>MSDTSPGPEHAPAIDRLLQIATGFMASKVLLVAASLGLFTELAAGPLRGEELRARLRLHPRSARDFFDTLVALGVLERTNGAYANTPATAQYLVRGKSAYLGGLLEMSDARMYELWGRLDEGLRTGNPQNEIRTGEEGIYATLYDDPDRLDAFQQAMTGLSMRSAHALAEAIDWSAYRTVADIGCAEGTVLIHLLERHPHLRGTGFDLAAVRPSFQRRHEESGLGDRLAFRAGDFFAEPLPQADALVFGHILSNWALPKAKTLLRKAHEALPEGGIVVIYETLIDDERRENVPGLLMSLTMLLETPGGFEYTGADCREWLADAGFRESRVQYLAGPESMVIATK[4x]

Among bisindoles, reductasporine is distinct due to its dimethylpyrrolinium structure. Its previously reported biosynthetic gene cluster encodes two unique tailoring enzymes, the imine reductase RedE and the dimethyltransferase RedM, which were shown to produce reductasporine from a common bisindole intermediate in recombinant E. coli. RedE reduces compound 4 to didemethylreductasporine, and then RedM catalyzes two methylations to give reductasporine. RedM is a homodimeric protein with monomers consisting of a largely α-helical N-terminal domain (α1-10, β1-3) and a Rossmann-like fold C-terminal domain (α12–16, β4-10) bridged by a long interdomain α-helix (α11). The C-terminal domain possesses a Rossmann-like fold typical of Class I SAM-dependent methyltransferases, with a β-sheet of five parallel strands terminated with two antiparallel strands each interspersed with α-helices.

The movement is an approximate 12° rotation toward α11 about an axis aligned with α15, where the loop regions around α15 act as flexible hinges. Helix α11 accommodates this conformational change by developing a kink at M157 or S161 with 31 to 49° changes in the Phi and Psi angles at these residues. The overall length of the monomer is reduced by 2.5 Å and the central binding cavity volume is reduced by up to 60% (estimated via POCASA), and likely represents a closed conformation of RedM. This conformation is seen in two protomer chains of the RedM-SAM structure: chains A and B. They adopt slightly different closed conformations with an average Cα displacement of 2.5 Å, rotating toward the dimerization domain about an axis roughly parallel with helix α8. Chains C and D have more open conformations similar to the unliganded and SAH-bound RedM structures. Upon closure of the active site, residues F153 and M157 from the interdomain helix α11 are brought to within 4 Å of the SAM methylsulfur, displacing the solvent. The two chains in the asymmetric unit of the RedM-SAM complex adopting closed conformations have higher B-factors along the periphery of the Rossmann-like domain compared to their dimer partners and corresponding weaker crystal symmetry contacts. In docking the substrate to the closed conformation several poses remain in this distal area, but higher-scoring poses occur near SAM.>MGASMTGGQQMGAPITAYAQQTRGLLGCIITSLTGRDKNQVEGEVQIVSTATQTFLATCINGVCWTVYHGAGTRTIASPKGPVIQMYTNVDQDLVGWPAPQGSRSLTPCTCGSSDLYLVTRHADVIPVR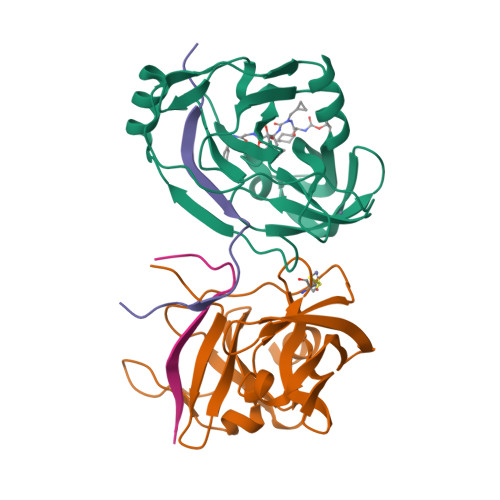RRGDSRGSLLSPRPISYLKGSSGGPLLCPAGHAVGLFRAAVCTRGVAKAVDFIPVENLETTMRSGSHHHHHH[2x];>KKGSVVIVGRIVLSGKPAIIPKK[2x]>[3x]VIRHFLRDDDLSPAEQAEVLELAAELKKDPVSRRPLQGPRGVAVIFDKNSTRTRFSFELGIAQLGGHAVVVDSGSTQLGRDETLQDTAKVLSRYVDAIVWRTFGQERLDAMASVATVPVINALSDEFHPCQVLADLQTIAERKGALRGLRLSYFGDGANNMAHSLLLGGVTAGIHVTVAAPEGFLPDPSVRAAAERRAQDTGASVTVTADAHAAAAGADVLVTDTWTSMGQENDGL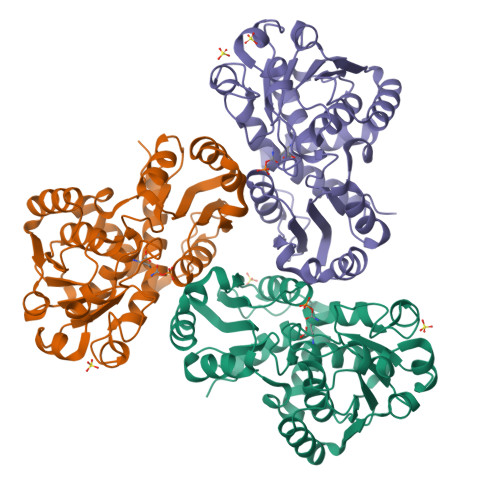DRVKPFRPFQLNSRLLALADSDAIVLHCLPAHRGDEITDAVMDGPASAVWDEAENRLHAQKALLVWLLERS> MRNLKRIVMGENKLIGLVRTALDSITLGQGVNEAKIKSPQSYAFHTISVGTISLDICKAIYSSSEIGRKQLENLSKKYNMPFEDLWFYGGFLHDWNKLSGKEESLENKEELTKKIIDKLKLPNEFLHGISTMAEGHLPDNLHLPLWVSIKLADMLLISDIGSVRDVFYFANSDSYRNAIEALKEYNLELNYVSSTFRLFTLIASKELLNDVFNEKSGYFPLISYADGIVFLKRKNSQPVLLSKIVDLLSRQVFSSSSEVIEEKISDIEKCIKNKEELFRQMNIDVKSAIYDEEGKVKQINAFLPTKVCKPFEDVVGNLDNKSKLQVAREVIERNRKDIPFGLLIYFVNKFSKNEEDYIRKGLGINEKSLKYLLNIGDVQKALDKILELLEKRYA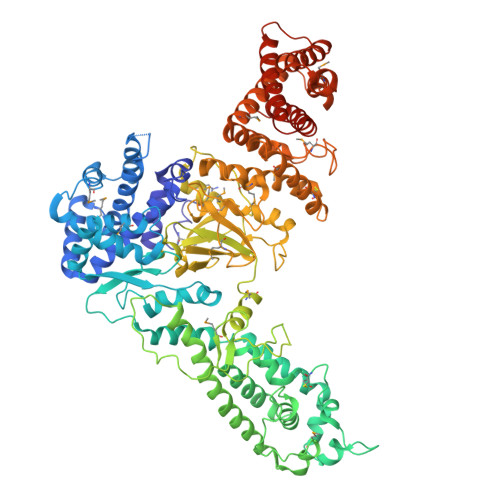EQSSDKTLLYYVKFSSSGNIIDDLPKITDRPNDYCVVCGMPIYSSNPVRFVQYASELGGRAEIWIPREKALDEIDNVRDDWKVCPICIYEANLMKDRVKPPYFIVTFYPGVPISLLNIIDFDFSQSSIKYYIDEEKDTYFTAFEKMGGRLEPYVKKVLPAYFSSKVIIKASEVSNFSLSTRLSKSELNKLLPYAPMISMIFLTSPVLISSNLYEMPIAHERVISITSTYNYTFMKSLNSNLLTLYSIFAYSAKYDAMRKICGRSDLDNCLGYLTEEMDLYSSVDPALGVLSIGMGVGTPIDTDEKFFSAFLPVSGYLLKVTGKVSKMGETLKSSIFSIAYALKDIIKSQKVSKYDVTGFLRDGVDMFFKTTSVIKDKEDRIGISVNAAISSLENKYALDDQHRAQVYSALQDIFKTLYSIEEESDRSLAISIANTLSNWLYIAYKLVLQGDKSLEHHHHHH3-(4-acetamidophenyl)benzoic acid | C15 H13 N O3 | 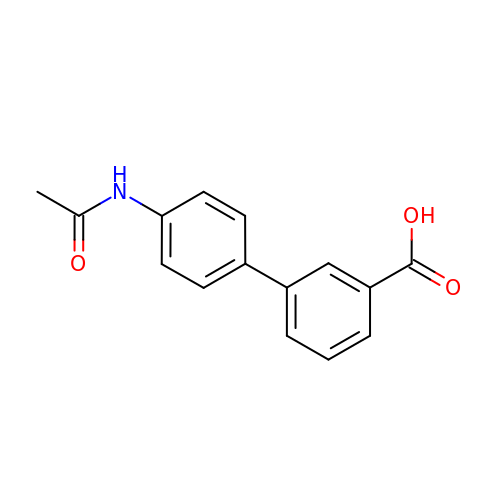ZIZLPMUXPKXCNP-UHFFFAOYSA-N>[2x]MGPQDNSLVIGASQEPRVLAGDFLRVISNQAIKSEIEQYLFAPFIGFNADSQNFPVLATEVPTLENGRLRVTDIGGGKKRLEMDITIRPDAKWSDGRPITTEDVAFYFEVGKAKGMPVLNPDFWERVNVRIKDARNFTLIFEPAYYYDTYGPINTYAPKHIMGPEWERVKAAARGLDPDKDAEKLNELYRNFFLKFATPQALNRGAMVYSGPFKLKRWVPGNSIEMERNPNFPIKPEGGESKYVQK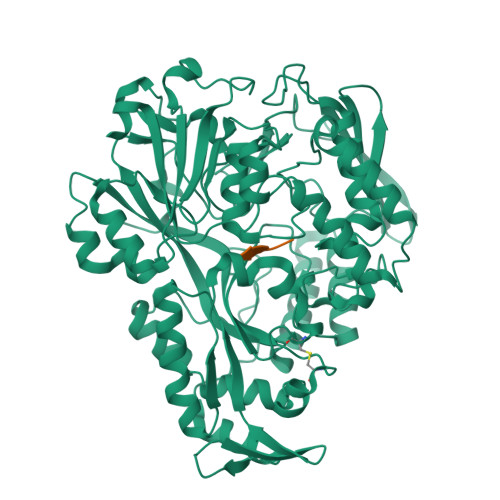VVYRFIQNTNSLLVAVIGGSIDATSSVSLTFDQGRSPQLVRRAPGRFDIWFVPGAIWEHIDINKFENCQVVKDLGLNDKRTRQAILHALNREGLVKAFFDGLQPVAHTWIAPVNPLFNPNVKKYEFDLKKAEALLAEMGWRKGPDGILQRTVNGRTVRFEIEYVTTAGNVVRERTQQFFAEDLKKIGIAVKINNAPSAVVFADEFIQRASECKWTGMFEFAWVSNLQEDGSLFQYKNLNTGAIMVPTKENNYQGQNIGGWRNDEFDRLTSQAVLEFDPERRKQLFWRAQEIWAEELPALPLYFRANPYVVRKGLVNYVASAYSGGYGYPGWNAWEIGWESRGAVKKWDQAKYALSTR;> ASKPK;> ASKTK Phosphotriesterase-like Lactonases (PLLs) are appealing candidates, being natural lactonases endowed with promiscuous phosphotriesterase activity. PTEs and PLLs belong to the amidohydrolase superfamily, and share the same (β/α)8 barrel topology. SsoPox exhibits high acyl-homoserine lactones and oxo-lactones hydrolysis abilities, and promiscuous, low phosphotriesterase activity. SsoPox is a very appealing candidate for the bioremediation of phosphotriesters because of its unique thermal stability, and its ability to resist aging, solvent and protease treatments.

Of them, the most active variants, αsA1 (C258L-I261F-W263A), αsA6 (F46L-C258A-W263M-I280T), αsB5 (V27A-I76T-Y97W-Y99F-L130P-L226V), αsC6 (L72I-Y99F-I122L-L228M-F229S-W263L), and αsD6 (V27A-Y97W-L228M-W263M) were subject to kinetic and structural characterization. The best improved variant, αsD6, exhibits a 2,210-fold increase in catalytic efficiency against methyl-parathion. Interestingly, some selected variants retained a strong preference for oxono-phosphotriesters (~10-fold), whereas others such as αsD6 lost the thiono-effect. Interestingly, the improved variants do not exhibit significant difference in KM values for thiono-phosphotriesters, but show a dramatic increase in kcat values, as compared to wild-type enzymes (e.g. kcat value of 6.89 s−1 and 1.10 × 10−3 s−1, as compared to methyl-parathion for the αsD6 variant and wild-type enzymes, respectively). The two selected variants, namely αsB5 and αsD6, which lost the thiono-effect have only two mutations in common: V27A and Y97W. Both residues are located relatively close to the bi-metallic active site, yet do not interact directly with the metals (V27-Fe: 6.7 Å, Y97-Co: 4.3 Å). While most structures were solved at high or medium resolutions (1.4–2.55 Å), mutant asD6 could only be solved at low resolution (2.95 Å). Given this resolution, we limited our interpretations and retained this data for the consistency of the study as it exhibits structural features (loop 8 disorder) that are consistent with all the other mutants. In the two other mutants, αsD6 and αsB5, loop 8 could not be modeled due to the lack of electronic density, which was likely to be due to the high level of motion of this enzyme region. Given both its catalytic proficiency and high thermal stability (Tm = 82.5 °C), αsD6 is a promising candidate for organophosphorus compound bioremediation and, in particular, the decontamination of water runoffs, soils, food products and materials.

>MRIPLVGKDSIESKDIGFTLIHEHLRAFSEAVRQQWPHLYNEDEEFRNAVNEVKRAMQFGVKTIVDPTVMGLGRDIRFMEKVVKATGINLVAGTGIWIYIDLPFYFLNRSIDEIADLFIHDIKEGIQGTLNKAGFVKIAADEPGITKDVEKVIRAAAIANKETKVPIITHSNAHNNTGLEQQRILTEEGVDPGKILIGHLGDTDNIDYIKKIADKGSFIGLDRYGLDMFLPVDKRNETTLRLIKDGYSDKIMISHDYCCTIDWGTAKPEYKPKLAPRWSITLIFEDTIPFLKRNGVNEEVIATIFKENPKKFFS[4x]>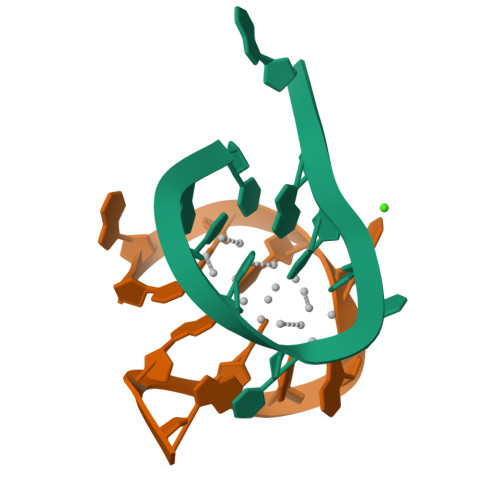[2x]CACCCAGCGA>KPPECPDFDPPRQENETWWLCDCFMATCKYNNTVEIVKVECEPPPMPTCSNGLQPVRVEDPDGCCWHWECDCYCTGWGDPHYVTFDGLYYSYQGNCTYVLVEEISPSVDNFGVYIDNYHCDPNDKVSCPRTLIVRHETQEVLIKTVHMMPMQVQVQVNRQAVALPYKKYGLEVYQSGINYVVDIPELGVLVSYNGLSFSVRLPYHRFGNNTKGQCGTCTNTTSDDCILPSGEIVSNCEAAADQWLVNDPSKPHCPHSSSTTKRPAVTVPGGGKTTPHKDCTPSPLCQLIKDSLFAQCHALVPPQHYYDACVFDSCFMPGSSLECASLQAYAALCAQQNICLDWRNHTHGACLVECPSHREYQACGPAEEPTCKSSSSQQNNTVLVEGCFCPEGTMNYAPGFDVCVKTCGCVGPDNVPREFGEHFEFDCKNCVCLEGGSGIICQPKRCSQKPVTHCVEDGTYLATEVNPADTCCNITVCKCNTSLCKEKPSVCPLGFEVKSKMVPGRCCPFYWCESKGVCVHGNAEYQPGSPVYSSKCQDCVCTDKVDNNTLLNVIACTHVPCNTSCSPGFELMEAPGECCKKC[2x]

The MUC2 mucin polymer is the main building unit of the intestinal mucus layers separating intestinal microbiota from the host epithelium. The MUC2 mucin is a large glycoprotein with a C-terminal domain similar to the MUC5AC and MUC5B mucins and the von Willebrand factor (VWF). The C-terminal part of MUC2 is made up by a VWD assembly, a series of VWC-domains and a C-terminal CK. A low-resolution image of the MUC2-C closely related MUC5B C-terminal has been published, but currently no high-resolution information is available for the mucins or VWF. Here, we present a model of the C-terminal part of MUC2 (MUC2-C) revealed by combining Cryo-EM and AlphaFold modeling which show an elongated dimer held together by covalent disulfide bonds in both ends.

Using Cryo-EM, it was possible to obtain structural information of MUC2-C from the VWCN domain to the VWC3 domain at an average resolution of 3.4 Å. The MUC2-C dimer model shows two regions: an N-terminus with a compact globular peptide chain and a C-terminal tail with the domains in tandem organized into a stalk that ends with the CK domain. The MUC2-C homodimer globular region in the N-terminal end presents a C2 symmetry, whereas the C-terminal tail had a non-regular double and twisted stalk conformation. The VWC1 is followed by VWC’, a truncated VWC domain, VWC3 and VWC4 domains and the C-terminal end with a typical CK domain. Our structural information shows that there is no VWB domain, but rather a serial repetition of VWC domains, disturbed by the truncated VWC’ domain only containing the C-leaf part and the two disulfide bonds acting as a knot. Interestingly, for all domains in MUC2-C the N-leaf subdomain mediates domain dimerization. The C-terminus of MUC2-C shows high flexibility due to several bending points. These are located between each VWC domain and within the Cys-knuckle subdomain. During particle selection and 3D volume reconstruction, this flexibility made it impossible to extend the map beyond VWC3 of the fully glycosylated MUC2-C. The Cryo-EM map loses intensity after the Cys-knuckle of VWC3.>[4x]MPKRTDIKSILILGAGPIVIGQACEFDYSGAQACKALREEGYRVINVNSNPATIMTDPEMADATYIEPIHWEVVRK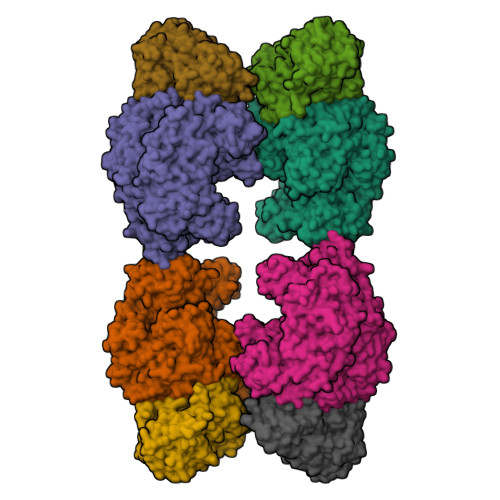IIEKERPDAVLPTMGGQTALNCALELERQGVLEEFGVTMIGATADAIDKAEDRRRFDVAMKKIGLETARSGIAHTMEEALAVAADVGFPCIIRPSFTMGGSGGGIAYNREEFEEICARGLDLSPTKELLIDESLIGWKEYEMEVVRDKNDNCIIVCSIENFDAMGIHTGDSITVAPAQTLTDKEYQIMRNASMAVLREIGVETGGSNVQFAVNPKNGRLIVIEMNPRVSRSSALASKATGFPIAKVAAKLAVGYTLDELMNDITGGRTPASFEPSIDYVVTKIPRFNFEKFAGANDRLTTQMKSVGEVMAIGRTQQESLQKALRGLEVGATGFDPKVSLDDPEALTKIRRELKDAGADRIWYIADAFRAGLSVDGVFNLTNIDRWFLVQIEELVRLEEKVAEVGITGLNADFLRQLKRKGFADARLAKLAGVREAEIRKLRDQYDLHPVYKRVDTCAAEFATDTAYMYSTYEEECEANPSTDREKIMVLGGGPNRIGQGIEFDYCCVHASLALREDGYETIMVNCNPETVSTDYDTSDRLYFEPVTLEDVLEIVRIEKPKGVIVQYGGQTPLKLARALEAAGVPVIGTSPDAIDRAEDRERFQHAVERLKLKQPANATVTAIEMAVEKAKEIGYPLVVRPSYVLGGRAMEIVYDEADLRRYFQTAVSVSNDAPVLLDHFLDDAVEVDVDAICDGEMVLIGGIMEHIEQAGVHSGDSACSLPAYTLSQEIQDVMRQQVQKLAFELQVRGLMNVQFAVKNNEVYLIEVNPRAARTVPFVSKATGVPLAKVAARVMAGKSLAEQGVTKEVIPPYYSVKEVVLPFNKFPGVDPLLGPEMRSTGEVMGVGRTFAEAFAKAQLGSNSTMKKHGRALLSVREGDKERVVDLAAKLLKQGFELDATHGTAIVLGEAGINPRLVNKVHEGRPHIQDRIKNGEYTYIINTTSGRRAIEDSRVIRRSALQYKVHYDTTLNGGFATAMALNADATEKVISVQEMHAQIK;>[4x]MIKSALLVLEDGTQFHGRAIGATGSAVGEVVFNTSMTGYQEILTDPSYSRQIVTLTYPHIGNVGTNDADEESSQVHAQGLVIRDLPLIASNFRNTEDLSSYLKRHNIVAIADIDTRKLTRLLREKGAQNGCIIAGDNPDAALALEKARAFPGLNGMDLAKEVTTAEAYSWTQGSWTLTGGLPQAKKEDELPFHVVAYDFGAKRNILRMLVDRGCRLTIVPAQTSAEDVLKMNPDGIFLSNGPGDPAPCDYAITAIQKFLETDIPVFGICLGHQLLALASGAKTVKMKFGHHGGNHPVKDVEKNVVMITAQNHGFAVDEATLPANLRVTHKSLFDGTLQGIHRTDKPAFSFQGHPEASPGPHDAAPLFDHFIELIEQYRKTAK> AVSFIGSTENDVGPSLGSYSRTHAMDNLPFVYDT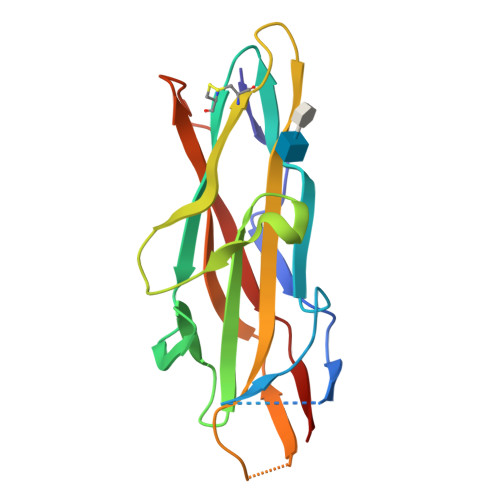RNKIGYQNANVWHISKGFCVGLDGKVDLPVVGSLDGQSIYGLTEEVGLLIWMGDTKYSRGTAMSGNSWENVFSGWCVGANTASTQGLSVRVTPVILKRNSSARYSVQKTSIGSIRMRPYNGSSAGSVQTTVNFSLNPFTLNDT> MNSTHHYEQLIEIFNSCFADEFNTRLIKGDDEPIYLPADAEVPYNRIVFAHGFYASAIHEISHWCIAGKARRELVDFGYWYCPDGRDAQTQSQFEDVEVKPQALDWLFCVAAGYPFNVSCDNLEGDFEPDRVVFQRRVHAQVMDYLANGIPERPARFIKALQNYYYTPELTAEQFPWPEALSLEHHH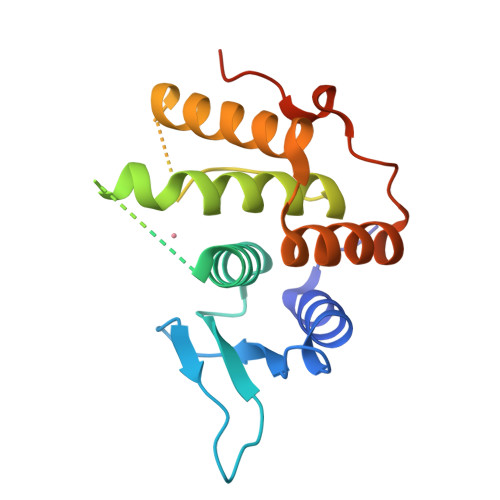HHH4-{(2S)-2-[2-(4-chlorophenyl)-5,6-difluoro-1H-benzimidazol-1-yl]-2-cyclohexylethoxy}benzoic 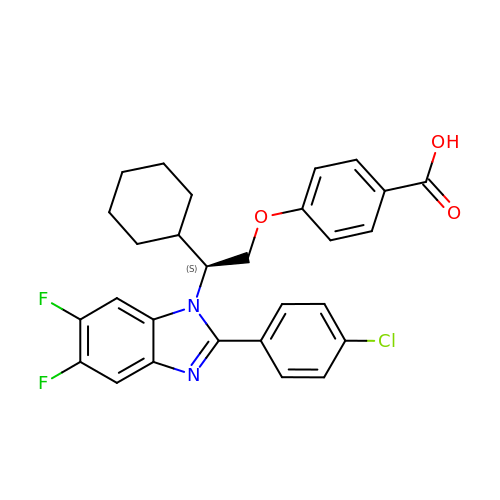acid | C28 H25 Cl F2 N2 O3 | DLAMZHRFSSYYFX-AREMUKBSSA-N>RSELRFDPGTSNRNFRIAASDFGQALMLPRLYATLEETAPQVRVTGVNLRHGPLVEELESGSIDIAFGGFPTLSAGIKTQTLFREEYVCVMRQSHPALTHGLDLEAFRQCRHIIVTAHEFNHVHEQVEARLLELLPPESIRFTTENFLVSAVIA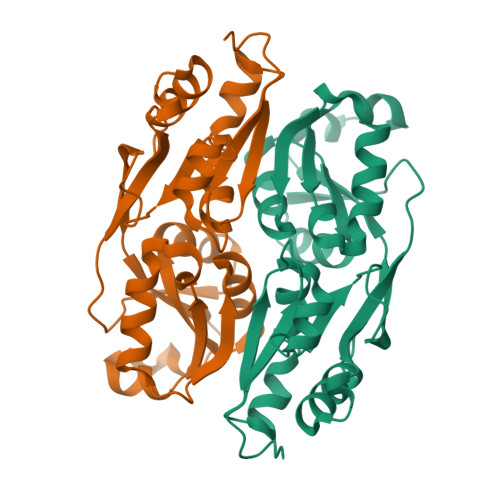EETDVILTIPSRLARWFANRGGLTIFPVPIELPSIEVKQYWHERYDKDPGNIWLRRVIAKIGFQNPPAE[4x]>[6x]AIERTFSIIKPNAVAKNVIGNIFARFEAAGFKIVGTKM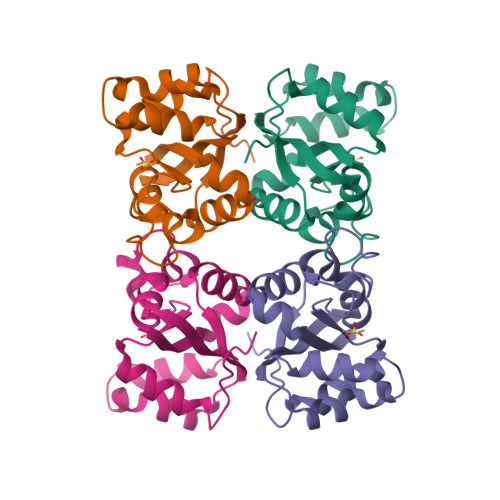LHLTVEQARGFYAEHDGKPFFDGLVEFMTSGPIVVSVLEGENAVQRHRDLLGATNPANALAGTLRADYADSLTENGTHGSDSVESAAREIAYFFGEGEVCPRTR5-[3-chloranyl-2-fluoranyl-6-(1,2,3,4-tetrazol-1-yl)phenyl]-2-[(1~{R})-2-cyclopropyl-1-[4-(2-methylpyrazol-3-yl)pyrazol-1-yl]ethyl]-1-oxidanyl-pyridine 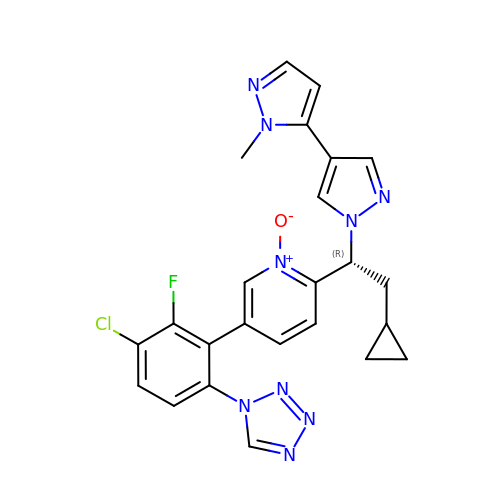| C24 H21 Cl F N9 O | DMOBSIYHBZREAR-JOCHJYFZSA-N>MPVRRGHVAPQNTFLDTIIRKFEGQSRKFIIANARVENCAVIYCNDGFCELCGYSRAEVMQRPCTCDFLHGPRTQRRAAAQIAQALLGAEERKVEIAFYRKDGSCFLCLVDVVPVKNEDGAVIMFILNFEVVMEKDMVGSPAHDTNHRGPPTSWLAPGRAKTFRLKLPALLALTARESSVRSGGAGGAGAPGAVVVDVDLTPAAPSSESLALDEVTAMDNHVAGLGPAEERRALVGPGSPPRSAPGQLPSPRAHSLNPDASGSSCSLARTRSRESCASVRRASSADDIEAMRAGVLPPPPRHASTGAMHPLRSGLLNSTSDSDLV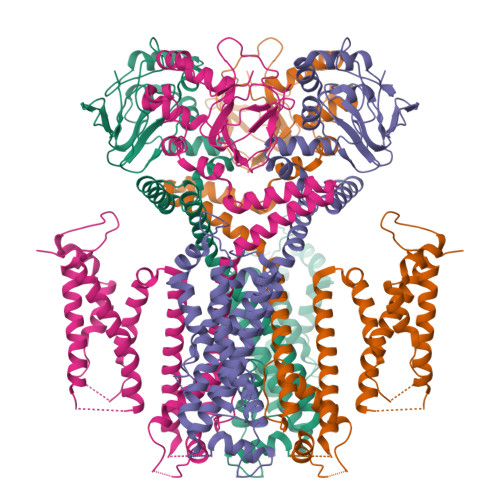RYRTISKIPQITLNFVDLKGDPFLASPTSDREIIAPKIKERTHNVTEKVTQVLSLGADVLPEYKLQAPRIHRWTILHYSPFKAVWDWLILLLVIYTAVFTPYSAAFLLKETEEGPPATECGYACQPLAVVDLIVDIMFIVDILINFRTTYVNANEEVVSHPGRIAVHYFKGWFLIDMVAAIPFDLLIFGSGSEELIGLLKTARLLRLVRVARKLDRYSEYGAAVLFLLMCTFALIAHWLACIWYAIGNMEQPHMDSRIGWLHNLGDQIGKPYNSSGLGGPSIKDKYVTALYFTFSSLTSVGFGNVSPNTNSEKIFSICVMLIGSLMYASIFGNVSAIIQRLYSGTARYHTQMLRVREFIRFHQIPNPLRQRLEEYFQHAWSYTNGIDMNAVLKGFPECLQADICLHLNRSLLQHCKPFRGATKGCLRALAMKFKTTHAPPGDTLVHAGDLLTALYFISRGSIEILRGDVVVAILGKNDIFGEPLNLYARPGKSNGDVRALTYCDLHKIHRDDLLEVLDMYPEFSDHFWSSLEITFNLRDTNMIPGSPGSTELEGGFSRQRKRKLSFRRRTDKDTEQPGEVSALGPGRAGAGPSSRGRPGGPWGESPSSGPSSPESSEDEGPGRSSSPLRLVPFSSPRPPGEPPGGEPLMEDCEKSSDTCNPLSGAFSGVSNIFSFWGDSRGRQYQELPRCPAPTPSLLNIPLSSPGRRPRGDVESRLDALQRQLNRLETRLSADMATVLQLLQRQMTLVPPAYSAVTTPGPGPTSTSPLLPVSPLPTLTLDSLSQVSQFMACEELPPGAPELPQEGPTRRLSLPGQLGALTSQPLHRHGSDPGS[4x]>MEVVKFMDVYQRSYCHPIETLVDIFQEYPDEIEYIFKPSCVPLMRCGGCCNDEGLECVPT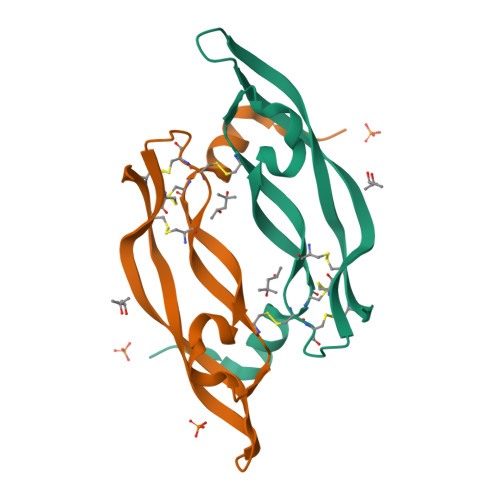EESNITMQIMRIKPHQGQHIGEMSFLQHNKCECRPK[2x]> ANTVNLQEAVA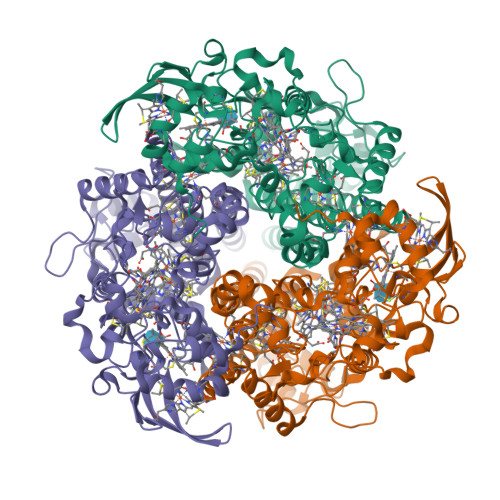KLKNVSPQTKTCLSCHISVTPGIVADWLKSKMAHVTPAEAWQKPALEREVSTPLDEIPANLRNVVVGCYECHGLNPEKHPDTIDHFGFKIHPIVTPNDCAVCHRTEVEQYSKSSKAWAYYNLMHNPIYRALVNASTMFTCMGKTFGGERTSQETSCLACHGTVVKVVGTVDTISHGIPVTLVKYEGYPNHGVGRVNPDGSLGACTACHPRHSFDIEIARSPYTCGQCHLDPDVPAFNVWKESKHGNIWFMHHKKYNMKAPAWKPGADFTAPTCATCHMSLLVNPVTGEVIAERTHNVDTRLWVRLFGLIYAHPMPRTGQHFKLSVEAMPESTAEALAKQGLTIAKALVGVKLPMPISLAPDIKTGKFLYATLPDGSPGLISEEEMAKRREQMVKICSACHNTEYAEYRMRLLDTQIEETNKATLKTTVLLLKAWQSGLAHVDLAKPVTLFDEYIEKLWVESWLFYSNSIRYGTAMNGQDWTTFKRGWYQLTKDIEHMKTLLRLWEAARAA>[2x]GPSGGGADVNKGPWAMALTPMEFARKYNLLRKDDALLDNPVPGEEMTAGIEEGDAKRVFTMQLGPYWDGFERCSPQAYALSAVFMARMNRDRDAANNILKVLDKTFVDGKPDFSVARPV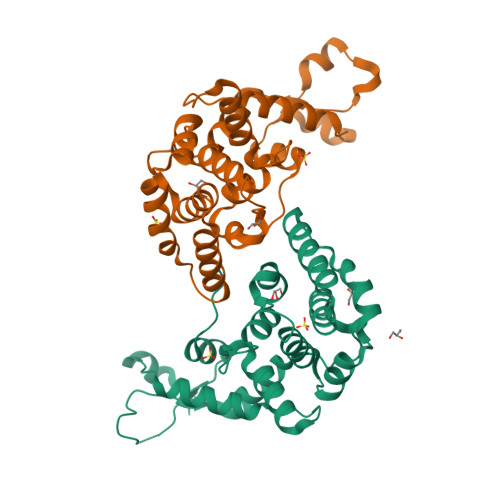MKKYQNSELVQEVVAKHAYVLTVIASLLEAAREDGVVPSSEFLWLKPVDRRLWYMLNCVGRQTPYSEVAGPFAHWKAEKEMGRRSLVPMIDEAIRALEIAVKEVRLTPRQMEELEP Bacterial β-lactamase enzymes are a major contributor to antibiotic resistance by hydrolyzing β-lactam antibiotics. Avibactam, which is used in combination with the β-lactam antibiotic ceftazidime, possesses a relatively broad-spectrum inhibition activity as it can inhibit class A, C, and some class D β-lactamases including extended-spectrum β-lactamases such as SHV variants. Furthermore, avibactam inhibits serine β-lactamases via a reversible mechanism which differentiates it from the currently available inhibitors. We found avibactam covalently bonded to S70 in the active site of KPC-2 and SHV-1.

KPC-2 hydrolyzes clavulanic acid, is phenotypically resistant to inhibitors and bacteria expressing this class A β-lactamase represent a major global health threat. The inhibition of KPC-2 by avibactam differs from the inhibition of other β-lactamases; avibactam, in addition to reversible deacylation, undergoes a slow desulfation. When bound to KPC-2, avibactam makes hydrogen bonds via its carbonyl oxygen in the oxyanion hole (comprised of backbone nitrogen atoms of S70 and T237), via the amide moiety with N132, and via its sulfate moiety with residues S130, T237, T235, and the main chain oxygen of T235. Residue W105, located 4.4 Å away is providing modest van der Waals interactions with the C4 atom of avibactam. In addition, K234 is potentially making a long range hydrogen bond electrostatic interaction with the sulfate moiety of avibactam with a distance of slightly greater than 3.3Å (not shown in Fig 4 due to cut-off 3.2Å distance used). The observed presence of the covalent bond involving S70 as well as the hydrogen bonding network between S130 and K73, and K234 and S70 are all conserved in CTX-M-15, SHV-1, and KPC-2 although the distance between S130 and K73 is somewhat larger in KPC-2 (3.35 Å) compared to the 2.8 Å and 3.1 Å distances observed in CTX-M-15 and SHV-1, respectively. The KPC-2:avibactam structure aids in explaining the structural basis of engineered substitutions that were shown to lead to resistance to this inhibitor against KPC-2. The second residue that impacts avibactam inhibition in KPC-2 is K234R. This change (K →R) has an intermediate effect on ampicillin/avibactam resistance; this side chain is hydrogen bonding to S130 in the KPC-2:avibactam structure. R220M is the third amino acid substitution in KPC-2 that has a modest effect on MIC (32 mg/L) compared to the other two changes. This is anticipated since this residue is not within hydrogen bonding distance of avibactam in the acyl complex structure, it is positioned more than 4 Å from the sulfate moiety, but could still have a significant electrostatic interaction with the negatively charged avibactam group. The chirality of N1 of avibactam is likely S in KPC-2 although the 1.8Å resolution of this structure is not sufficient to assign this chirality with 100% confidence; in the other β-lactamases, it is either R or planar.

> TNLVAEPFAKLEQDFGGSIGVYAMDTGSGATVSYRAEERFPLCSSFKGFLAAAVLARSQQQAGLLDTPIRYGKNALVPWSPISEKYLTTGMTVAELSAAAVQYSDNAAANLLLKELGGPAGLTAFMRSIGDTTFRLDRWELELNSAIPGDARDTSSPRAVTESLQKLTLGSALAAPQRQQFVDWLKGNTTGNHRIRAAVPADWAVGDKTGTCGVYGTANDYAVVWPTGRAPIVLAVYTRAPNKDDKHSEAVIAAAARLALEGLG> SGSSEQELAAIVRDLGCGPYFLGTHDKRFPGFLAGNKLACAIVNTAGRETG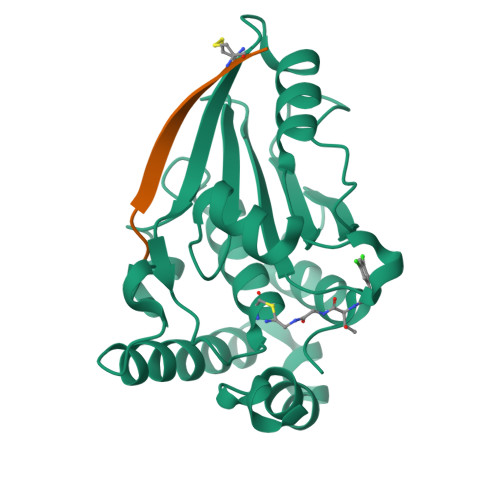GVHWLAFGWNPRSRTCYMFDPFGFSDRRLKQIYSFEYEAMLRRSALALSPDRCLSLEQSTQTVQGPDSAACGLFCCMFLHAFVHWPDRPMDGNPTMNLLTGVPNGMLQSPQVLPTLRRNQEKLYRFLAHHSPYFRSHRAAIEHATAFDKMKQL;> GVKSLKRRRCY>MSLAVKPGEPLPDFLLLDPKGQPVTPATVSKPAVIVFWASWCTVCKAEFPGLHRVAEETGVPFYVISREPRDTREVVLEYMKTYPRFIPLLASDRDRPHEVAARFKVLGQPWTFVVDREGKV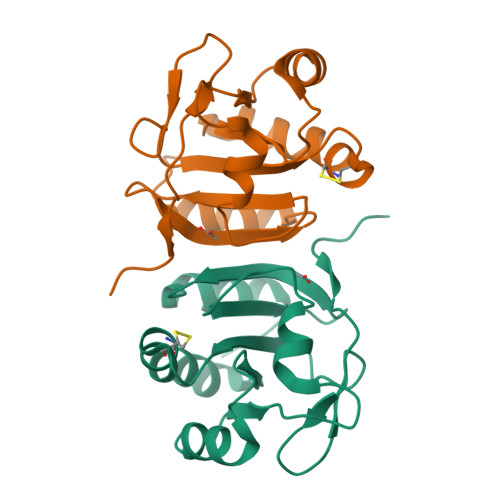VALFAGRAGREALLDALLLAGADLEGHHHHHH[2x]1-[(4~{S})-9-propan-2-ylsulfonyl-1-oxa-9-azaspiro[5.5]undecan-4-yl]-3-[[4-(trifluoromethyloxy)phenyl]methyl]urea 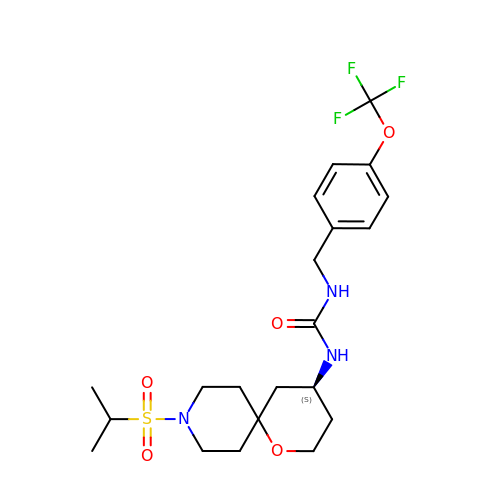| C21 H30 F3 N3 O5 S | BZTKUYQNORQBRG-KRWDZBQOSA-N> HMFEARLVQGSILKKVLEALKDLINEACWDISSSGVNLQSMDSSHVSLVQLTLRSEGFDTYRCDRNLAMGVNLTSMSKILKCAGNEDIITLRAEDNADTLALVFEAPNQEKVSDYEMKLMDLDVEQLGIPEQEYSCVVKMPSGEFARICRDLSHIGDAVVISCAKDGVKFSASGELGNGNIKLSQT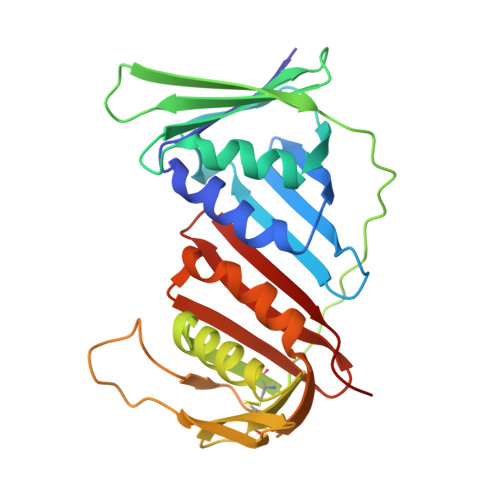SNVDKEEEAVTIEMNEPVQLTFALRYLNFFTKATPLSSTVTLSMSADVPLVVEYKIADMGHLKYYLAPKI6-fluoro-1,3-benzothiazol-2-amine | C7 H5 F N2 S | 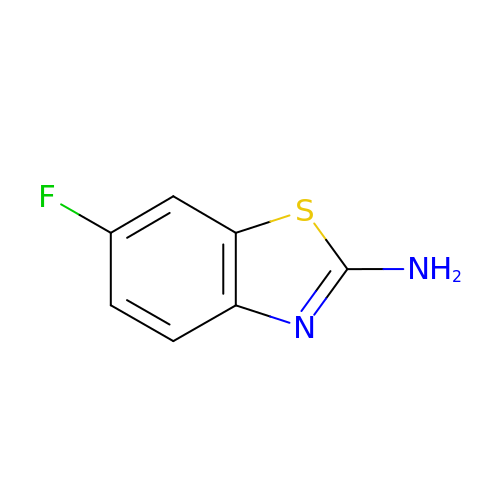CJLUXPZQUXVJNF-UHFFFAOYSA-N>[6x]GSHMGTEDLKYSLERLREILERLEENPSEKQIVEAIRAIVENNAQIVEAIRAIVENNAQIVEILRAIIEALEAIGVDQKILEEMKKLLKDLKRSLERG

We used de novo protein design to generate very closely related proteins that adopt two very different states—a short state and a long state, like a viral fusion protein—and then created a single molecule that can be found in both forms. Inspired by class I viral fusion proteins, such as influenza hemagglutinin, we chose homotrimeric helical bundles as the fundamental architecture. We decided on a design scheme with two divergent conformations containing a constant six-helix bundle “base” and a variable portion with three inner helices and three “flipping” helices. In the compact “short” state (∼66 Å height), the flipping helices fold back to interact with the inner helices; in the extended “long” state (∼100 Å height), they extend to form interactions with each other.

The interaction energy between the flipping helix and the inner helices in the short state was tuned by combining hydrogen bond layers (“A”) or hydrophobic layers (“X”) in different orders in each of three possible positions. Designs were given three-letter names corresponding to the layers in order, starting at the hinge proximal position. We sought to design calcium- or nickel-binding sites in the long state by introducing aspartic acid or histidine at the key hinge residue position. We also designed for structural ambiguity in the turn—with the result that the secondary structure prediction for residue 75 is mixed helical and coil, but with low confidence. Crystal structures were determined for all potential bistable candidates (XAX_GGDQ, XXA_GVDQ, XAA_GGHN, and XAA_GVDQ), and we chose to focus on XAA_GVDQ because of the presence of a bound calcium.l-asparaginase II (EC 3.5.1.1) is an amidohydrolase that primarily catalyzes the hydrolysis of l-Asn to l-Asp and ammonia, but that can also act on other substrates, including l-Gln. This enzyme has been used for over 40 years in the treatment of leukemias, particularly Acute Lymphoblastic Leukemia (ALL), which is the most prevalent cancer in childhood. Many studies focus on the EcA2 from the K12 strain (EcA2-K12), which differs by four amino acids from reference biopharmaceuticals, including Elspar (EcA2-4M). To understand the structural implications of the four-amino acid differences between EcA2-K12 and EcA2-4M, we solved their crystal structure in the presence of l-Asp under the same crystallization condition and data collection method.

All monomers in the asymmetric unit showed the l-Asp in the active site. The monomers of EcA2-K12 and EcA2-4M were essentially superposable, with Cα RMSD values lower than 0.4 Å. The structural and comparative analysis of EcA2-4M and EcA2-K12 showed a good correspondence between the positions of nonmatching residues and their electron density maps, with the only exception being the valine at position 27 of EcA2-K12. There was poor correspondence between the electron density map and the spatial position of valine 27, which may be due to the characteristics of the added residue and its location in EcA2-K12. Given its hydrophobicity and constant interaction with a highly solvated region, vital for the opening and closing mechanism of the active site loop, this may lead to greater dynamics compared to alanine 27 of EcA2-4M. Additionally, among the amino acid sequence differences between EcA2-K12 and EcA2-4M, only the amino acid at position 27 is located within the enzyme active site (Val27 in K12 and Ala27 in 4M), more precisely in the N-terminal flexible loop. The much lower catalytic efficiency of EcA2-K12 for l-Gln, which has an extra CH2 group in its side chain compared to l-Asn, is likely due to steric hindrance caused by the bulkier side chain of the valine at position 27 compared to the alanine in EcA2-4M, which allows better accommodation of l-Gln. However, considering the turnover rates, the EcA2-K12 variant is more specific for l-Asn, with a k cat Asn/k cat Gln ratio of 66.7 ± 0.2. However, for the EcA2-K12 variant, the disappearance of the Tyr25 resonances is only observed in the presence of >600 μM of l-Asp. Our data indicate that EcA2-K12 has lower activity due to the higher conformational dynamics of the N-terminal active site loop.

>[4x]LPNITILATGGTIAGGGDSATKSNYTVGKVGVENLVNAVPQLKDIANVKGEQVVNIGSQDMNDNVWLTLAKKINTDCDKTDGFVITHGTDTMEETAYFLDLTVKCDKPVVMVGAMRPSTSMSADGPFNLYNAVVTAADKASANRGVLVVMNDTVLDGRDVTKTNTTDVATFKSVNYGPLGYIHNGKIDYQRTPARKHTSDTPFDVSKLNELPKVGIVYNYANASDLPAKALVDAGYDGIVSAGVGNGNLYKSVFDTLATAAKTGTAVVRSSRVPTGATTQDAEVDDAKYGFVASGTLNPQKARVLLQLALTQTKDPQQIQQIFNQY> SNAMRSAQVYRWQIPMDAGVVLRDRRLKTRDGLYVCLRDGEREGWGEISPLPGFSQETWEEAQTALLTWVNDWLQGSEGLPEMPSVAFGASCALAELTGVLPEAADYRAAPLCTGDPDDLVLRLADMPGEKIAKVKVGLYEAVRDGMVVNLLLEAIPDLHLRLDANRAWTPLKAQQFAKYVNPDYRAR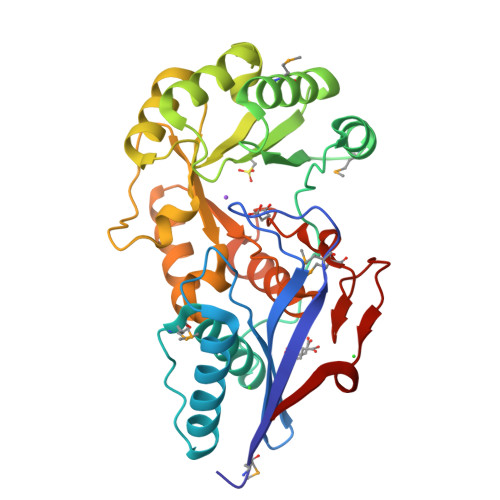IAFLEEPCKTRDDSRAFARETGIAIAWDESLREADFTFEAEEGVRAVVIKPTLTGSLDKVREQVAAAHALGLTAVISSSIESSLGLTQLARIAAWLTPGTLPGLDTLHLMQAQQIRPWPGSALPCLKREELERLL>[2x]RAMDYKDDDDKLRSLLVWTGEPTTKHFSDIFLGRCLIYTQILRPEMRDQNCQEILSTFKGAFVSKNPCDITREDYAPLVKLVTQTIPCDKTLFWSKSKHLAHQYTWIQGKMFTLEDTLLGYIADDLRWCGDPSTSDMNYVSCPHWSENCPNNPITMFWKVI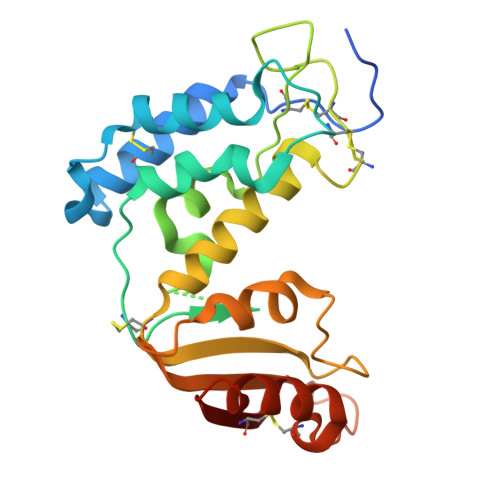SQKFAEDACGVVQVMLDGSLREPFYKDSTFGSVEVFSLDPNKVHKLQAWVMHDIEGASSNACSSSSLNELKMIVQKRNMIFACVDNYRPARF>[2x]GAMDRPGPPEGPVVISGVTAEKCTLAWKPPLQDGGSDIINYIVERRETSRLVWTVVDANVQTLSCKVTKLLEGNEYTFRIMAVNKYGVGEPLESEPVVAKNPFVVPDAPKAPEVTTVTKDSMIVVWERPASDGGSEILGYVLEKRDKEGIRWTRCHKRLIGELRLRVTGLIENHDYEFRVSAENAA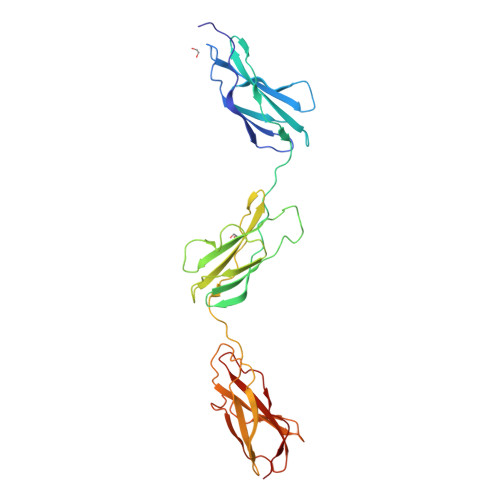GLSEPSPPSAYQKACDPIYKPGPPNNPKVIDITRSSVFLSWSKPIYDGGCEIQGYIVEKCDVSVGEWTMCTPPTGINKTNIEVEKLLEKHEYNFRICAINKAGVGEHADVPGPIIVEE> ARKCSLTGKWTNDLGSNMTIGAVNSKGEFTGTYTTAVTATSNEIKESPLHGTQNTINKRTQPTFGFT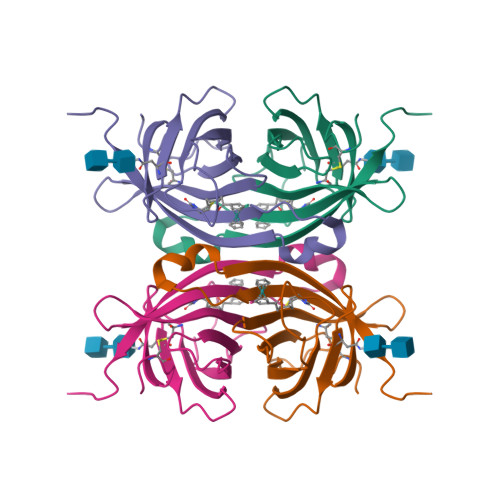VNWKFSESTTVFTGQCFIDRNGKEVLKTMWLLRSSVNDIGDDWKATRVGINIFTRLRTQKE>MRLSYEALEWRTPIENSTEPVSLPPPPPFFGQERAREALELAIRGGFHAYLVGPPSLGKHEALLAYLSTQSVETPPDLLYVPLSERKVAVLTLPSGQEIHLAEAVEGLLLEVNRLDELFRQGSFLREKTQLEARFKEAREQQLEALRREAQEAGFALSTNGERLELTGPGPVPAELSARLEEVTLGSLAASAELEVALRRLRRDWALHYLNNRFEPLFQRFPQARAYLEALRARLARYAETGEPLDPAQWRPNLLTSSSSGTPPPIVYEPYATAPRLFGRLDYLVDRGVWSTNVSLIRPGAVHRAQGGYLILDALSLKREGTWEAFKRALRNGQVEPVTEPQAPAGLEVEPFPIQMQVILVGTPEAFEGLEEDPAFSELFRIRAEFSPTLPASPENCTALGGWLLAQGFQLTQGGLTRLYDEARRMAEQRDRMDARLVEIRALAEEAAVLGGGLLTAESVEQAIAAREHRSFL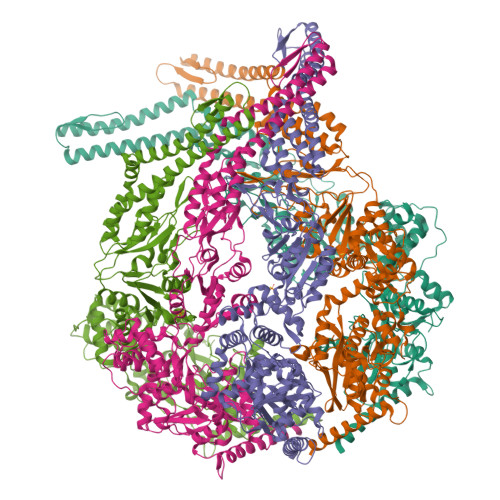SEEEFLRAVQEGVIRLRTTGRAVGEVNSLVVVEAAPYWGRPARLTARAAPGRDHLISIDREAGLGGQIFHKAVLTLAGYLRSRYIEHGSLPVTISLAFEQNYVSIEGDAAGLAELVAALSAIGNLPLRQDLAVTGAVDQTGKVLAVGAINAKVEGFFRVCKALGLSGTQGVILPEANLANLTLRAEVLEAVRAGQFHIYAVETAEQALEILAGARMEGFRGLQEKIRAGLEAFARLEEGHDKEDREKLAAALEHHHHHH[5x]>AMADYDTYVSNVQINNLSYGVYTSGGKETQFFCIGLKHGSEAISINAMCKVDVYGNHKQGFDNML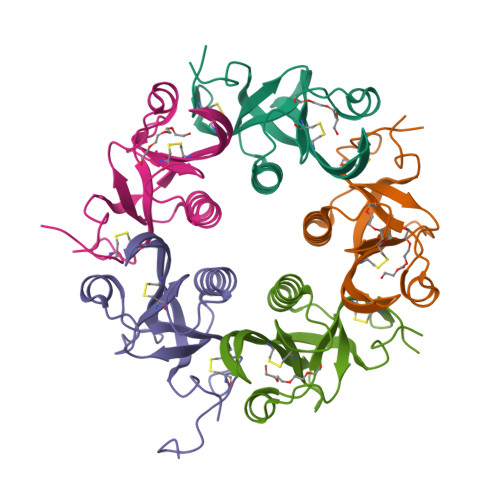NTAKYYYTTGGDVRIYYKENVWRDPDFKSAFSSRELIAITTCSSSSYCMGPTVTNLESD[5x]> PPK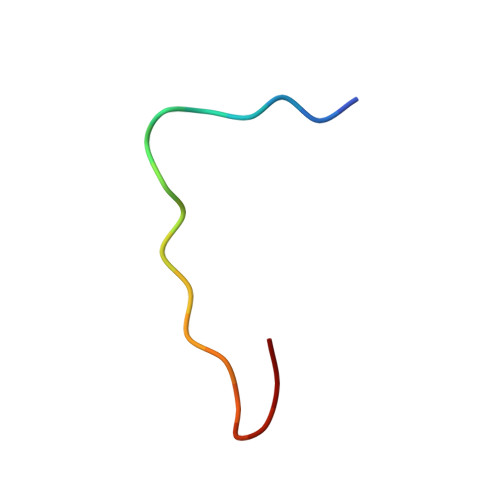RRAISAIRKFPRDCG>[24x]TEKTPDDVFKL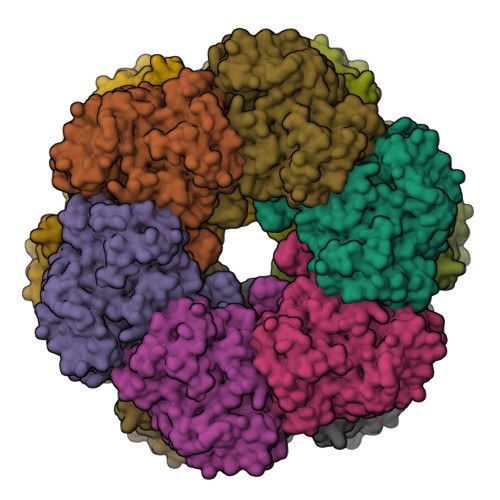AKDEKVEYVDVRFCDLPGIMQHFTIPASAFDKSVFDDGLAFDGSSIRGFQSIHESDMLLLPDPETARIDPFRAAKTLNINFFVHDPFTLEPYSRDPRNIARKAENYLISTGIADTAYFGAEAEFYIFDSVSFDSRANGSFYEVDAISGWWNTGAATEADGSPNRGYKVRHKGGYFPVAPNDQYVDLRDKMLTNLINSGFILEKGHHEVGSGGQAEINYQFNSLLHAADDMQLYKYIIKNTAWQNGKTVTFMPKPLFGDNGSGMHCHQSLWKDGAPLMYDETGYAGLSDTARHYIGGLLHHAPSLLAFTNPTVNSYKRLVPGYEAPINLVYSQRNRSACVRIPITGSNPKAKRLEFRSPDSSGNPYLAFSAMLMAGLDGIKNKIEPQAPVDKDLYELPPEEAASIPQTPTQLSDVIDRLEADHEYLTEGGVFTNDLIETWISFKRENEIEPVNIRPHPYEFALYYDV> GSNPNDLPDFPEHEYAATQQVGEGVINGDLYLTSASGAIQKGTNTKVALEPATSYMKAYYAKFGNLDAAKRDPDVQPPVLDPRRATYVREATTDQ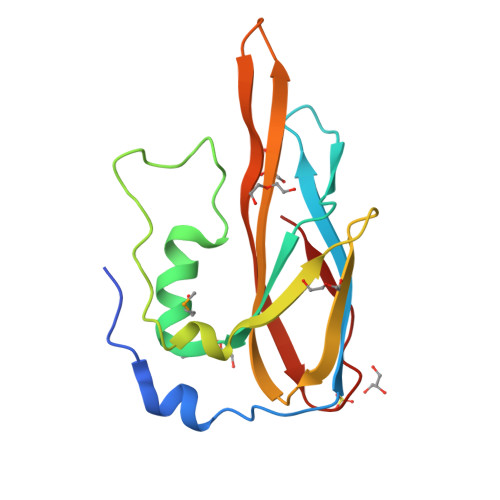NGRFDFDHIPNGTYYISSELTWSAQSDGKTITEGGTVTKLVTVSGSQPQKVLLTR> MNVTIYDVAREASVSMATVSRVVNGNPNVKPSTRKKVLETIERLGYRPNAVARGLASKKTTTVGVIIPDISNIFYAELARGIEDIATMYKYNIILSNSDQNQDKELHLLNNMLGKQVDGIIFMSGNVTEEHVEELKKSPVPVVLAASIESTNQIPSVTIDYEQAAFDAVQSLI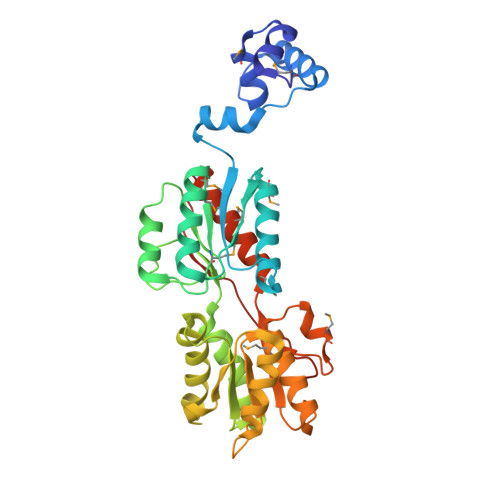DSGHKNIAFVSGTLEEPINHAKKVKGYKRALTESGLPVRDSYIVEGDYTYDSGIEAVEKLLEEDEKPTAIFVGTDEMALGVIHGAQDRGLNVPNDLEIIGFDNTRLSTMVRPQLTSVVQPMYDIGAVAMRLLTKYMNKETVDSSIVQLPHRIEFRQSTK> GSAEIIRCS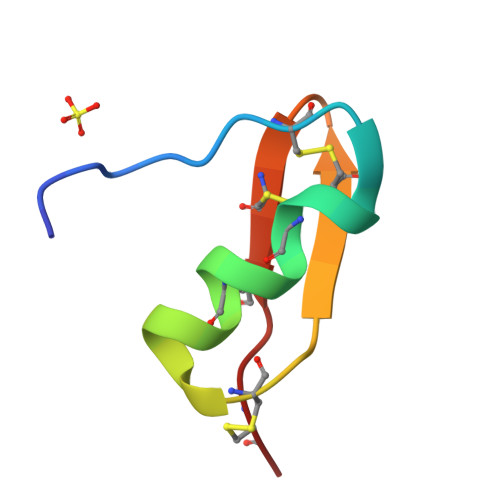GTRECYAPCQKLTGCLNAKCMNKACKCYGCV>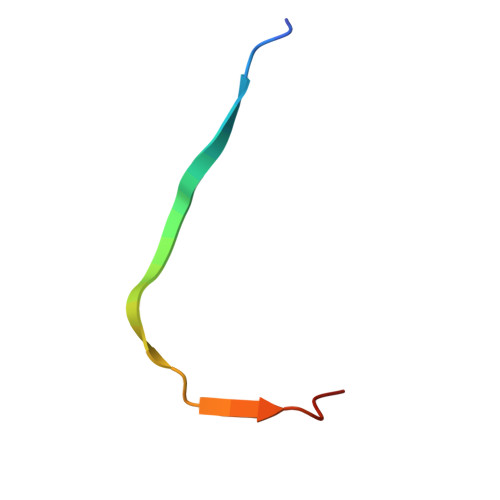 AGSMIRTMLQGKLHRVKVTHADLHYEG>[2x]MAPTAIEHMEPPFWWAGMQHKGLQLMVHGRDIGRMEAALDYPGVRLVSTTRVPNANYLFVDLEIGPEAQPGSFDIVFKGDGRSERYRYRLLAREQGSAQRQGFGPGDAIYQIMPDRFANGDPSNDNVAGMREQADRRHGGGRHGGDIRGTIDHLDYIAGLGFTQLWPTPLVENDAAAYSYHGYAATDHYRIDPRYGSNEDFVRLSTEARKRGMGLIQDVVLSHIGKHHWWMKDLPTPDWINYGGKFVPTQHHRVAVQDPYAAQADSENFTKGWFVEGMPDLNQTNPLVANYLIQNNIWWIEYAGLSGLRIDTYGYSDGAFLTEYTRRLMAEYPRLNMVGEEWSTRVPVVARWQRGKANFDGYTSHLPSLMDFPLVDAMRNALSKTGEENGLNEVYETLSLDYLYPEPQNLVLFGGNHDMARMFSAAGEDFDRWRMNLVFLMTMPRIPQFYSGDEILMTSTVKGRDDASYRRDFPGGWAGDKANAFSGA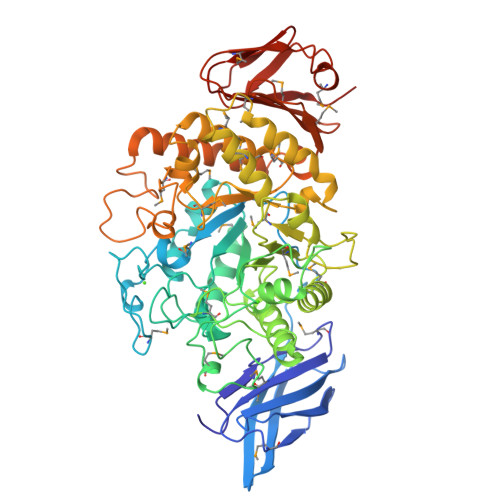GLTSQQRAAQDLVRKLANWRKNQPVIHNGRLMHFGPEENTWVYFRYNKDKRIMVAMNNNDKPMTLPTARFQEMLKGAPSGVDFLSGKTVGLGRELRLAPKSVVVIELPGLPEA Clostridioides difficile causes life-threatening gastrointestinal infections. Herein, we report 30 X-ray structures from a structure genomics pipeline spanning 13 years, representing 10.2% of the X-ray structures for this important pathogen. The Center for Structural Biology of Infectious Diseases (CSBID, formerly the Center for Structural Genomics of Infectious Diseases) implemented a structural biology pipeline starting in 2010 through paired efforts with systems biology, bioinformatics, and other research specialists in C. difficile pathogenesis. This project ultimately involved 335 proteins linked with pathogenesis, metabolism, and antimicrobial resistance.

The structures presented here are part of the C. difficile 630, R20291, and Y384 sets nominated at CSBID.

> MKTSSNASITDGNGNYSIAGATYGVFADKDCTKQLATLTTNENGNTDVVEVTTGTVYIRELSAPAGYKVDKTVYSLKVEAGKTATLKVSDTPKVTDTLIELFKIDMETQKDNPQGNASLAGAEFTWKYYAGFYNKENLPAEATRTWVTKTIAETDSDGTTHYITKLADAYKVSGDSFYMQDGKAVLPLGTLTVEETKAPNGYLLDGAYMQAGDKSEQIKGLYVTQITEDGDLAVLSGSNQFSVSDKVIRGGVKIQKRDLETGDTKPQGSATLKDTAFDIISLNDNVVLVEGKLYKKNEVVKTIHTDIEGVASTSADLLPYGKFRIVESEAPNGYLTDGAKPIDFAITENGKIVDLTDEAHSGAAL>GMTPLDANVELPTEVKAMIEQSSDAQAATALV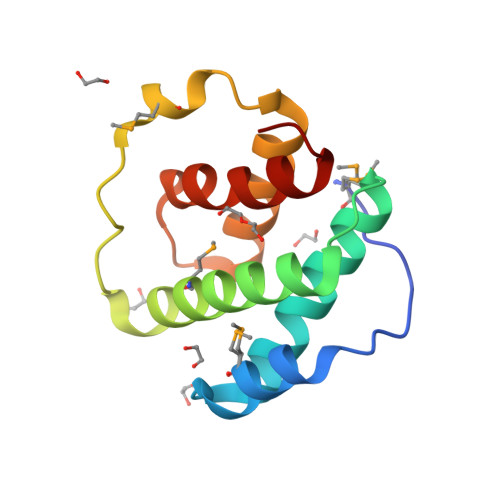NYVIKLAAAAEIHFTDLQLQVLTNHLIEMLGRSKSGEQLPAVDPTMFAEVSQKSLDLADQVVQHIGHLEVAEKYVLSIHFEAAQDKI[2x]>GSATATTRMFKTIDARRSQHLDLGGSLVGPESVAFDGKGRGPYSGVSDGRIMRWNGEAAGWSTYTYSPSYTKNKCAASTLPTVQTESKCGRPLGLRFHYKTGNLYIADAYMGLMRVGPKGGEATVLAMKADGVPLRFTNGVDIDQVTGDVYFTDSSMNYQRSQHEQVTATKDSTGRLMKYDPRTNQVTVLQSNITYPNGVAMSADRTHLIVALTGPCKLMRHWIRGPKTGKSEPFVDLPGYPDNVRPDGKGGYWIALHREKYELPFGPDSHLVAMRVSAGGKLVQQMRGPKSLRPTEVMERKDGKIYMGNVELPYVGVVKSS[12x]

An indole-3-acetic acid (IAA)-glucose hydrolase, THOUSAND-GRAIN WEIGHT 6 (TGW6), negatively regulates the grain weight in rice. Ishimaru and Hirotsu et al. first identified THOUSAND-GRAIN WEIGHT 6 (TGW6), a gene that limits the number of endosperm cells and rice grain weight. An enzyme activity assay confirmed the IAA-Glc hydrolase activity of TGW6 using recombinant TGW610. From another point of view, the hydrolysis of IAA glycoconjugates by TGW6 has been considered to function in auxin metabolism.

The crystal structure of TGW6 was determined at 2.6 Å resolution and exhibited a six-bladed β-propeller structure. The Root Mean Square Deviation (RMSD) of the corresponding atomic positions in 12 molecules were calculated less than 0.5 Å by the DALI server. According to the result of structural similarity search, the structure of TGW6 was classified into six-bladed β-propeller structure. Furthermore, some proteins with structural similarity to TGW6, such as diisopropylfluorophosphatase (DFPase), gluconolactonase (XC5397)23 and drug resistance protein 35 (Drp35), retain calcium (Ca2+). In contrast, the highly conserved Ca2+-binding motif in structurally similar proteins was not completely conserved in TGW6, and a Ca atom was not found at the site using single-wavelength anomalous diffraction. Therefore, these results implied that the Ca2+ ion does not bind at the partially conserved Ca2+-binding site in TGW6 or that the binding affinity was very weak even if the ion interacted. Thermal shift assays revealed that TGW6 preferably interacted with indole compounds among the tested substrates, enzyme products and their analogs. Firstly, the docking pose of IAA-Glc was simulated when the IAA portion of the chemical structure bound to the inside of the molecule around phenylalanine (Phe)-165, histidine (His)-192 and tyrosine (Tyr)-224 in TGW6 (subpocket A; the interior portion of the nipped pocket), whereas that of Glc interacted at the site relatively close to the molecular surface around Glu-193, arginine (Arg)-287 and Glu-343 (subpocket B; the outer portion of the nipped pocket). Notably, the IAA moiety bound to fill the shape of subpocket A, whereas subpocket B still had a vacant space. The interaction map of IAA-Glc in the presence of TGW6 suggested that Tyr-224 was involved with hydrogen bonds, His-192 and His-286 interacted as aromatic-aromatic contacts, and Leu-121, Phe-165, His-286, threonine (Thr)-324 and valine (Val)-339 were engaged in hydrophobic interaction with the IAA substructure.>[6x]MGVISDAYRLKYTFGVDFGTSYVKYGPITLNEPKMVQTRGLFLRDLPESVKMRIPPDVLARGLVVGDEEVRKYLSSVRDVQRNLKYPLKDGVARRDDEEAWRVLKELARYTLAQFPVSDPEFAGWLVAVALSALAPDYMYKAIFDIYDELASEFKIYAVTILPQPLAVAIAENAVNCVIVEGGHGNIQVAPISFALIREGLVALNRGGAEANAITREI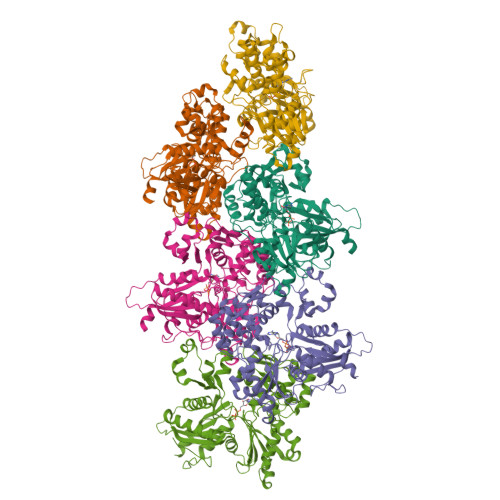LKDIGYSDIAREEYAVEVVKRAVGLVPRRLKEAIRAAKSDPDRFVTKVRLSPVVEVEIPREYAWTRFLIGEIVFDPNHEEIKSYIEQSRLRIENAVIGDVTLYGEMDVASAIITSLRNVSVEIQERVASQIILSGGAFSWRVPPGMEDVAADSVTRVKIALEEKSPALASKVEVRLVSEPQYSVWRGAVIYGYALPLSLEWSDTTREGWRFPRR> MEPGSVENLSIVYRSRDFLVVNKHWDVRIDSKAWRETLTLQKQLRYRFPELADPDTCYGFRFCHQLDFSTSGALCVALNKAAAGSAYRCFKERRVTKAYLALLRGHIQESRVTISHAIGRNSTEGRAHTMCIEGSQGCENPKPSLTDLVVLEHGLYAGDPVSKVLLKPLTGRTHQLRVHCSALGHPVVGDLT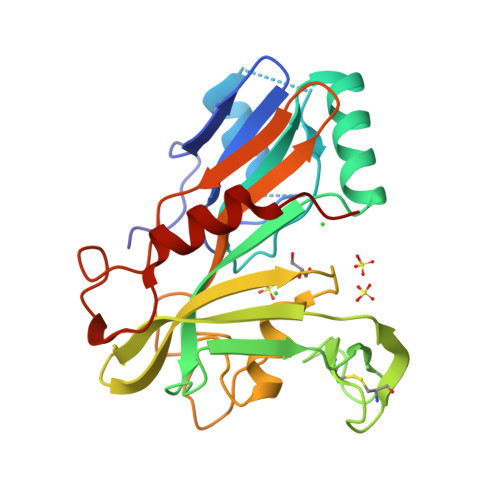YGEVSGREDRPFRMMLHAFYLRIPTDTECVEVCTPDPFLPSLDACWSPHTLLQSLDQLVQALRATPDPD>MAHHHHHHMKTLYTIGATATGGRN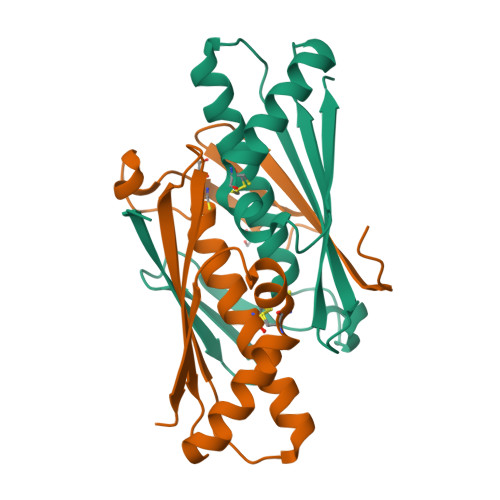GHVKSDNGVLEFEVRYPKGLGGANDDYANPEMLFAAGYSACFDSALNLVIKSAKIKTGETTVTAKVGIGQIENGGFGLEVELHANIPGVTIEEAQDLIEKAHQVCPYSNATRGNIEVKLTVSNN[2x]>[2x]GSGPAFESYESMELACPAERSGHVAVSDGRHMFVWGGYKSNQVRGLYDFYLPREELWIYNMETGRWKKINTEGDVPPSMSGSCAVCVDRVLYLFGGHHSRGNTNKFYMLDSRSTDRVLQWERIDCQGIPPSSKDKLGVWVYKNKLIFFGGYGYLPEDKVLGTFEFDETSFWNSSHPRGWNDHVHILDTETFTWSQPITTGKAPSPRAAH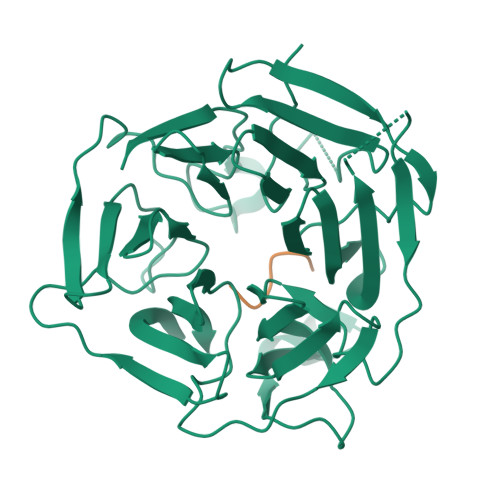ACATVGNRGFVFGGRYRDARMNDLHYLNLDTWEWNELIPQGICPVGRSWHSLTPVSSDHLFLFGGFTTDKQPLSDAWTYCISKNEWIQFNHPYTEKPRLWHTACASDEGEVIVFGGCANNLLVHHRAAHSNEILIFSVQP;>[2x]NQRFGSNNTSGS>[2x]MSFNTI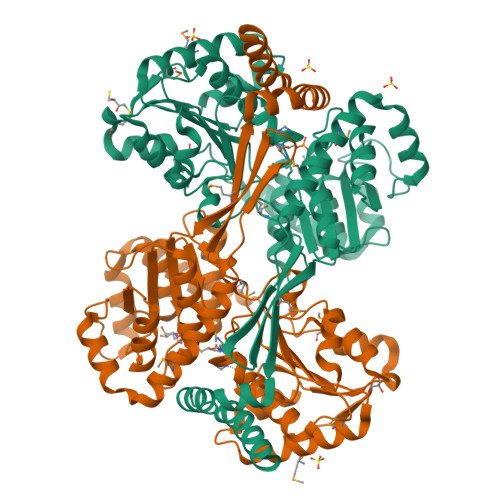IDWNSCTAEQQRQLLMRPAISASESITRTVNDILDNVKARGDEALREYSAKFDKTTVTALKVSAEEIAAASERLSDELKQAMAVAVKNIETFHTAQKLPPVDVETQPGVRCQQVTRPVASVGLYIPGGSAPLFSTVLMLATPASIAGCKKVVLCSPPPIADEILYAAQLCGVQDVFNVGGAQAIAALAFGTESVPKVDKIFGPGNAFVTEAKRQVSQRLDGAAIDMPAGPSEVLVIADSGATPDFVASDLLSQAEHGPDSQVILLTPAADMARRVAEAVERQLAELPRAETARQALNASRLIVTKDLAQCVEISNQYGPEHLIIQTRNARELVDSITSAGSVFLGDWSPESAGDYASGTNHVLPTYGYTATCSSLGLADFQKRMTVQELSKEGFSALASTIETLAAAERLTAHKNAVTLRVNALKEQA>MVLDVTKDHWLPYVLLAQLPVMVLFRKDNDEEAKKVEYIVRELAQEFDGLIRVFYVDINKAPEIAKKY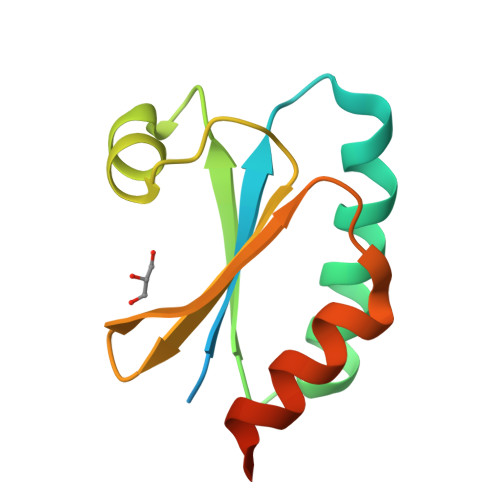NITTTPTVAFFHNGELKSVFTGAITKDQLRDEILKYLGLEHHHHHH[2x]>GHMSTLLINQPQYAWLKELGLREENEGVYNGSWGGRGEVITTYCPANNEPIARVRQASVADYEETVKKAREAWKIWADIPAPKRGEIVRQIGDALREKIQVLGSLVSLEMGKILVEGVGEVQEYVDICDYAVGLSRMIGGPILPSERSGH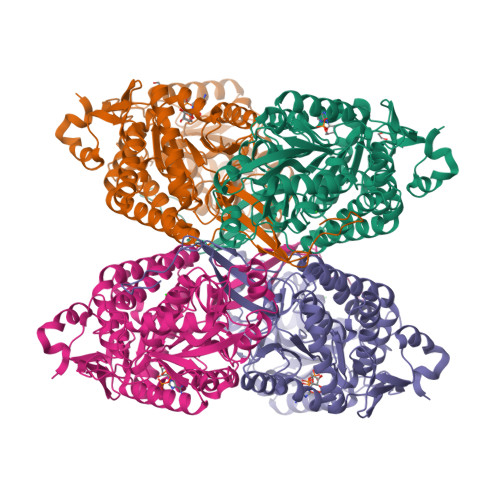ALIEQWNPVGLVGIITAFNFPVAVYGWNNAIAMICGNVCLWKGAPTTSLISVAVTKIIAKVLEDNKLPGAICSLTCGGADIGTAMAKDERVNLLSFTGSTQVGKQVGLMVQERFGRSLLELGGNNAIIAFEDADLSLVVPSALFAAVGTAGQRCTTARRLFIHESIHDEVVNRLKKAYAQIRVGNPWDPNVLYGPLHTKQAVSMFLGAVEEAKKEGGTVVYGGKVMDRPGNYVEPTIVTGLGHDASIAHTQTFAPILYVFKFKNEEEVFAWNNEVKQGLSSSIFTKDLGRIFRWLGPKGSDCGIVNVNIPTSGAEIGGAFGGEKHTGGGRESGSDAWKQYMRRSTCTINYSKDLPLAQGIKFQ[8x]>MKNVLIIFGKPYCSICENVSDAVEELKSEYDILHVDILSFFLKDGDSSMLGDVKRGTLIGNFAAHLSNYIV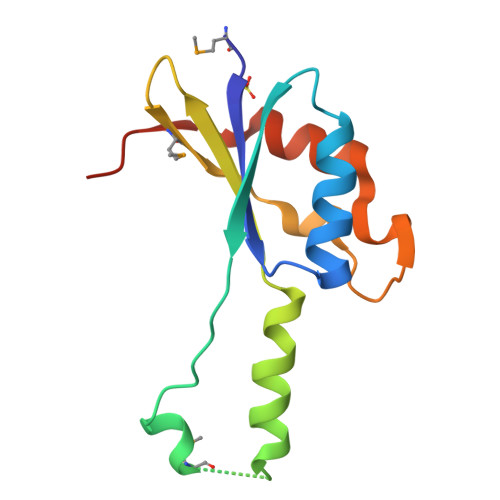SIFKYNPQTKQMAFVDINKSLDFTKTDKSLVNLEILKSEIEKATYGVWPPVTE[3x]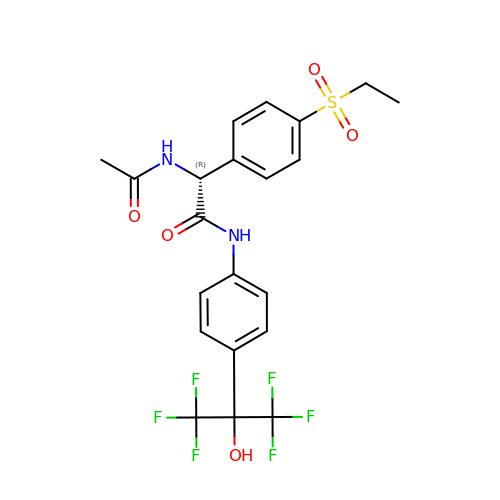(2~{R})-2-acetamido-2-(4-ethylsulfonylphenyl)-~{N}-[4-[1,1,1,3,3,3-hexakis(fluoranyl)-2-oxidanyl-propan-2-yl]phenyl]ethanamide | C21 H20 F6 N2 O5 S | HJJYGXDBXQAVQG-QGZVFWFLSA-N>[2x]EFHMEQKTPKESDRCGGCGKFTHEDDLIALEEEKKKEKEKPLMSKKKSHHHKKNDFQWIGCDSCQTWYHFLCSGLEQFEYYLYEKFFCPKCVPHTGHSIRYKVVAPHRYRWYSPNEKHLGIEVGSKTWIEDFITRENTVPSPTDDEVCIVEDGYEFRREFEKLGGADNWGKVFMVKDMDGLNMTMPKPGFDLEDVVKIMGSDYEVDTIDVYNQS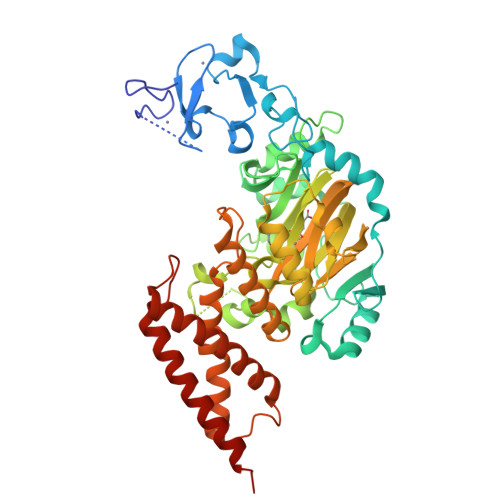TYSMKLDTFRKLFRDTKNRPLLYNFLSLEFSDNNEMKEIAKPPRFVQEISMVNRLWPDVSGAEYIKLLQREEYLPEDQRPKVEQFCLAGMAGSYTDFHVDFGGSSVYYHILKGEKIFYIAAPTEQNFAAYQAHETSPDTTTWFGDIANGAVKRVVIKEGQTLLIPAGWIHAVLTPVDSLVFGGNFLHLGNLEMQMRVYHLENAIRKEIRSEEKFYFPNFELLHWMYMRNVLLEKITEANQEGSDMREQEKNIWTASQIMKAEMERWMDRELRLGPEKNAILPTDDKNKIMISVRKQIEIQTKIQNAKNKPMGLK> GAMVTNHEQVLTDYLAAFIEELVQAGVKEAIISPGSRSTPLALMMAEHPILKIYVDVDERSAGFFALGLAKASKRPVVLLCTSGTAAANYFPAVAEANLSQIPLIVLTADRPHELRNVGAPQAMDQLHLYGSHVKDFTDMALPENSEEMLRYAKWHGSRAVDIAMKTPRGPVHLNFPLREPLVPILEPSPFTATGKKHHHVHIYYTHEVLDDSSIQKMVTECTGKKGVFVVGPIDKKELEQPMVDLAKKLGWPILADPLSGLRSYGALDEVVIDQYDAFLKEAEILDKLTPEVVIRFGSMPVSKPLKNWLEQLSDIRFYVVDPGAAWKDPIKAVTDMIHCDERFLLDIMQQNMPDDAKDAAWLSRWTSYNKVAREIVLAEMANTTILEEGKIVAELRRLLPDKAGLFIGNSMPIRDVDTYFSQIDKKIKMLANRGANGIDGVVSSALGASVVFQPMFLLIGDLSFYHDMNGLLMAKKYKMNLTIVIVNNDGGGIFSFLPQANEPKYFESLFGTSTELDFRFAAAFYDADYHEAKSVDELEEAIDKASYHKGLDIIEVKTNRHENKANHQALWAKIADALKALN

The ThDP-dependent enzyme 2-succinyl-5-enolpyruvyl-6-hydroxy-3-cyclohexene-1-carboxylate (SEPHCHC) synthase (MenD) catalyses the first irreversible step in bacterial classical menaquinone biosynthesis via a series of reactions involving covalent ThDP-bound intermediates. An important player in menaquinone production is the thiamine diphosphate (ThDP)-dependent decarboxylase MenD [2-succinyl-5-enolpyruvyl-6-hydroxy-3-cyclohexene-1-carboxylate (SEPHCHC) synthase]. MenD catalyses the first irreversible step of the classical menaquinone-biosynthesis pathway via two covalent ThDP intermediates; decarboxylation of 2-oxoglutarate produces intermediate I, with subsequent addition of isochorismate generating intermediate II and breakdown to release SEPHCHC. Analysis of the structures revealed that LmoMenD adopts the typical three-domain ThDP-dependent fold observed for MenD orthologs, while a combination of structure, size-exclusion chromatography, mass photometry and small-angle X-ray scattering analysis showed that the enzyme has a homotetrameric quaternary structure.

Analysis of the ThDP-bound LmoMenD structure suggests that the active-site configuration and ThDP-binding interactions are similar to those observed in other MenD enzymes. The ThDP diphosphate group tethers the cofactor to the enzyme via interactions with a divalent magnesium cation and the PP domain; specifically, residues Ser408, Met409, Asp459, Leu460 and Ser461, as well as Asn486 and Ile491, from the region that closes on the active site. The conserved residue Glu56 is likely to be involved in tautomerization of the aminopyrimidine ring during catalysis, and Ile436 is likely to be responsible for the bent ThDP conformation important for ThDP activation and catalysis, while Gln119 has speculative roles in many steps, including product release. Upon the application of crystallographic symmetry, a tetramer composed of a dimer of dimers is formed. Similarly, the ThDP-bound and intermediate I-bound structures (space group P6422) form the same dimer-of-dimers arrangement upon the application of crystallographic symmetry to the monomer present in the asymmetric unit. Comparison with a previously deposited but unpublished apo structure of LmoMenD revealed changes in key regions, resulting in a more closed active site in ligand-bound structures.>GGGRMDAATTRVGLTDLTFRLLRESFADAVSWVAKNLPARPAVPVLSGVLLTGSDNGLTISGFDYEVSAEAQVGAEIVSPGSVLVSGRLLSDITRALPNKPVDVHVEGNRVALTCGNARFSLPTMPVEDYPTLPTLPEETGLLPAELFAEAISQVAIAAGRDDTLPMLTGIRVEILGETVVLAATDRFRLAVRELKWSASSPDIEAAVLVPAKTLAEAAKAGIGGSDVRLSLGTGPGVGKDGLLGISGNGKRSTTRLLDAEFPKFRQLLPTEHTAVATMDVAELIEAIKLVALVADRGAQVRMEFADGSVRLSAGADDVGRAEEDLVVDYAGEPLTIAFNPTYLTDGLSSLRSERVSFGFTTAGKPALLRPVSGDDRPVAGLNGNGPFPAV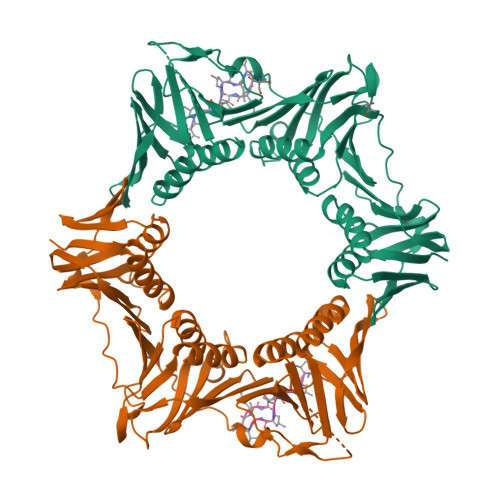STDYVYLLMPVRLPG[2x];>XVPTLPLVPXG[2x]N-DODECYL-N,N-DIMETHYLGLYCINATE 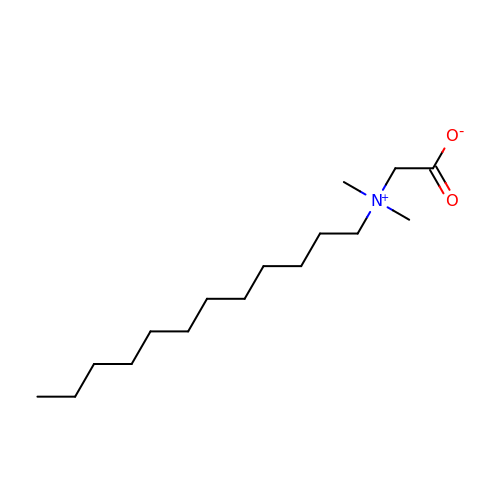| C16 H33 N O2 | DVEKCXOJTLDBFE-UHFFFAOYSA-N>GPGGEDVIDSLQLNELLNAGEYKIGELTFQSIRSSQELQKKNTIVNLFGIVK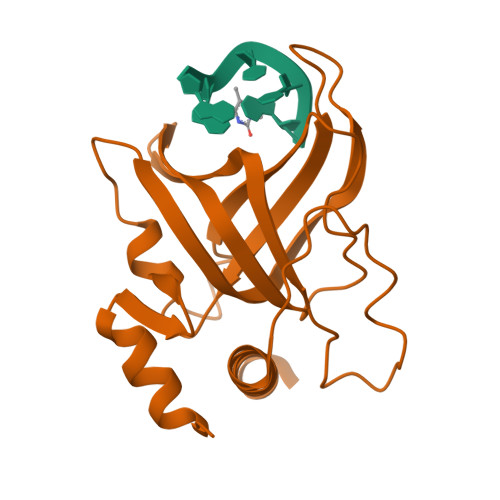DFTPSRQSLHGTKDWVTTVYLWDPTCDTSSIGLQIHLFSKQGNDLPVIKQVGQPLLLHQITLRSYRDRTQGLSKDQFRYALWPDFSSNSKDTLCPQPMPRLMKTGDKEEQFALLLNKIWDEQTNKHKNGELLSTS[2x]>PFTLPNLPLSSLSNSRAPLPISSMGISPDNVQSVQFQNGRCTLDGRLVGTTPVSLSHVAKIRGTSNGTVINLTELDGTPFHPFEGPAPIGFPDLGGCDWHINMTQFGHSSQTQYDVDTTPDTFVPHLGSIQANGIGSGNYVGVLSWISPPSHPSGSQVDLWKIPNYGSSITEATHLAPSVYPPGFGEVLVFFMSKMPGPGAYNLPCLLPQEYISHLASEQAPTVGEAALLHYVDPDTGRNLGEFKAYPDGFLTCVPNGASSGPQQLPINGVFVFVSWVSRFYQLKPVGTASSARGRLG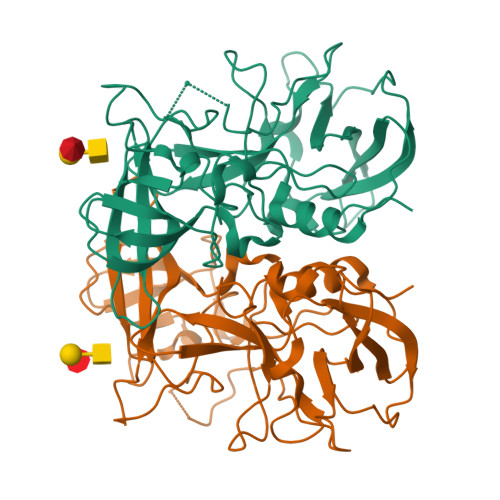LRR[2x]>SAPAPNVPGGERVCAYTSGLSSLSYASARVTYPCTLSKAAYPATTLTGGFSNTKEQMTWLSEHLSSHGYIVITITPRNIFGAPTGWESAHKAGIAKLRSERSRRASPLYNKLDPSKFALTGFSMGGGGALLAAADLGSQVKVAVPM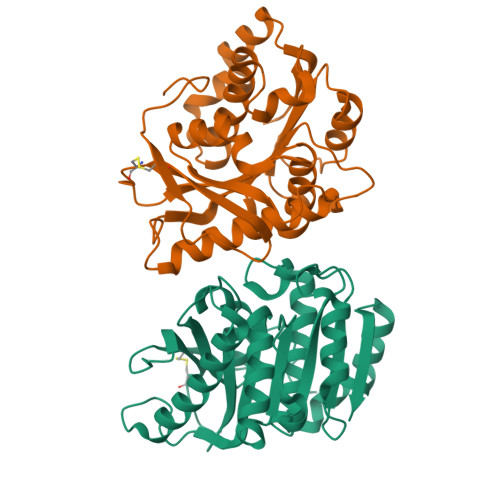APFLGSNNPNYSAITAKVLIQAGANDTVANPSTVASYYQSLPTGISRALTTFRSASHLDWINTGNTNRQARLKTLVTSWLKVYLDGNSDYATYLDGAEHSRHLAEDWFTRFEYVR[2x]>[2x]SQHNILEALNVRVVGTGDRILFLAHGFGTDQSAWHLILPYFTQNYRVVLYDLVCAGSVNPDYFDFNRYTTLDPYVDDLLNIVDSLGIQNCAYVGHSVSAMIGIIASIRRPELFSKLILIGFSPRFLNDEDYHGGFEEGEIEKVFSAMEANYEAWVHGFAPLAVGADVPAAVREFSRTLFNMRPDISLFVSRTVFNSDL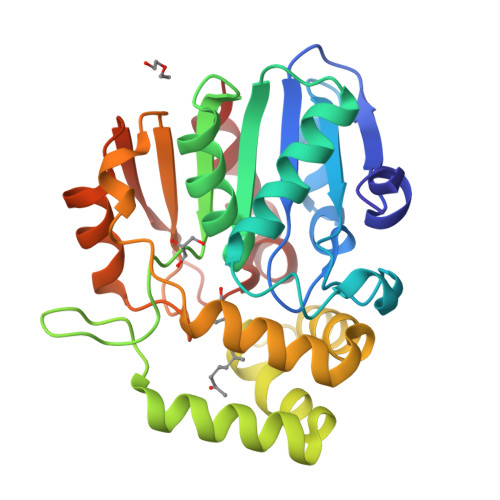RGVLGLVRVPTCVIQTAKDVSVPASVAEYLRSHLGGDTTVETLKTEGHLPQLSAPAQLAQFLRRALP> A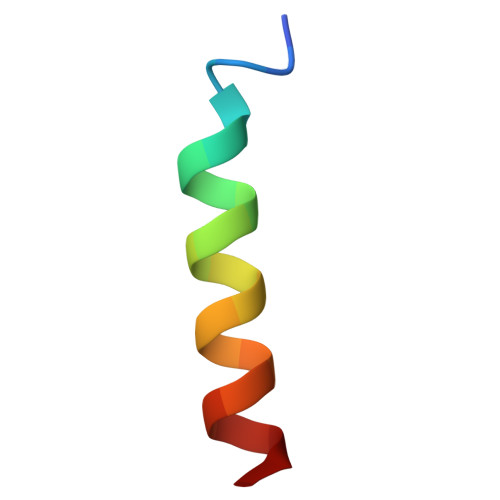AAAARAARAAAWRAEQAAAA Here we identified Vip3Cb1 and Vip3Cc1, the first Vip3 proteins with broad lepidopteran activity discovered outside of Bt from Paenibacillus strains in the P. popilliae-containing clade, most closely linked to P. dendritiformis. Vip3 proteins, including Vip3Cb1 and Vip3Cc1, are highly conserved in Domains (D) I and II involved in pore formation, with divergence in DIII, IV, and V known to be involved in receptor binding to the gut of the insect host. Vip3Cb1 protoxin and trypsin-processed Vip3Cb1 toxin structures were determined using Cryo-EM, resulting in density maps with an estimated resolution of 2.6 Å and 3.0 Å, respectively. Therefore, structural comparisons of Vip3Cb1 to other Vip3 proteins, including commercial Vip3Aa, are consistent with other results, such as amino acid homology, that all Vip3 proteins share the same mechanism of action, even though these originated from a Paenibacillus strain and not from Bt.

Artificial trypsin digestion mimics Vip3 activation by serine proteases abundant in lepidopteran midgut. The Vip3Cb1 N-terminus has the signature Vip3A signal peptide “ALPSF” motif. Upon activation with trypsin, cleavage occurs preferentially at Lysine 195; yet, the tetramer stays intact and undergoes large conformational changes, revealing a pore structure as determined by Cryo-EM (Fig. 4D through F). Although the extreme N-terminus density is lacking in the Cryo-EM density maps, modeling from Leu98 in DI is possible. The protoxin’s DI and N-terminal DII unfurl and rearrange into an extended 4 α-helical channel (α1act), while domains DIII-DV remain unchanged. The former protoxin α10 helix h2 leading into α5 (residues E205–V220) shifts down, becoming a more ordered α3act upon activation. In addition, protoxin α4 (residues 165–192) also moves down, becoming part of the newly formed channel α1act. At Pro168, there is a 63o bend in α1act which leads into the long-extended 4α-helical channel. The activated Vip3Cb1 quaternary structure is also like activated structures determined for Vip3Aa16 and Vip3Bc1, with large conformational changes in DI-II forming a long, extended α-helical channel. Vip3Cb1act tryptic site boundary modeling revealed density for the N-terminal 20 kDa fragment up to Asp185, and density resumed for the C-terminal 65 kDa fragment at Asn209, containing DII-V. Detection of a magnesium ion in the Vip3Cb1 channel is evidence that Vip3Cb1 can function as a pore for ions, causing osmotic imbalance and insect cell death. This magnesium ion was also observed in the Vip3Aa16act structure, similarly coordinated by the Asn (N163) side chain with a similar bond length (3.6 Å), and this Asn residue is highly conserved in Vip3 sequences.

>[4x]MHHHHHHHHHHGTETVRFQSKQNNNFSVRALPSFIDVFNGIYGFATGIQDIFNMIFGTDTGDLTLEEVLKNQELLYDISGKLEGISGDLSEIIAQGNLNTELAKELLKIANEQNNVLTDVNNKLNAINSMLHIYLPKITNMLSDVMKQNYALSLQIEYLSKQLQEISDKLDVINLNVLINSTLTEITPAYQRIKYVNEKFDELTLATEKTLRAKQGSEDIIANDTLENLTELTELAKSVTKNDMDSFEFYLHTFHDVLIGNNLFGRSALKTAAELITKDEIKTSGSEIGKVYSFLIVLTCLQAKAFLTLTACRKLLGLSDIDYTNILNQHLNDEKNVFRDNILPTLSNKFSNPNYVKTIGSDNYAKVILEAEPGYALVGFEIINDRIPVLKAYKAKLKQNYQVDHQSLSEIVYLDIDKLFCPKNSEQKYYTKSLTFPDGYVITKITFEKKLNNLRYEATANFYDPSTGDIDLNEKQVESTFLQADYISINVSDDDGVYMPLGVISETFLSPINSFELEVDEKSKILTLTCKSYLREYLLESDLINKETSLIAPPNVFISNIVENWNIEADNLEPWVANNKNAYVDSTGGIEGSKALFTQGDGEFSQFIGDKLKPNTDYIIQYTVKGKPAIYLKNKNTGYTMYEDTNGSSEEFQTIAVNYTSETDPSQTHLVFKSQSGYEAWGDNFIILECKAFETPEGPELIKFDDWISFGTTYIRDDVLTIDPSRGGYFRQSLKLDSYSTYNLSFSFSGLWAKVIIKNSHGVVLFEKVSQQSSYVDISESFTTTSNKEGFFIELTGDSRGGFGSFRDFSMKEKFE>[6x]TESDRIAGIFNIPAGIIPTGNVLSTIEVCAHRCIFDFFKQIRSDDNSLYSAQFDILLGTYCNTLNFVRFLELGLSVACICTKFPELAYVRDGVIQFEVQQPMIARDGPHPVDQPVHNYMVKRIHKRSLSAAFAIASEALSLLSNTYVDGTEIDSSLRIRAIQQMARNLRTVLDSFERGTADQLLGVLLEKAPPLSLLSPINKFQPEGHLNRVARAALLSDLKRRVCADMFFMTRHAREPRLISAYLSDMVSCTQPSVMVSRITHTNTRGRQVDGVLVTTATLKRQLLQGILQIDDTAADVPVTYGEMVLQGTNLVTALVMGKAVRGMDDVARHLLDITDPNTLNIPSIPPQSNSDSTTAGLPVNARVPADLVIVGDKLVFLEALERRVYQATRVAYPLIGNIDITFIMPMGVFQANSMDRYTRHAGDFSTVSEQDPRQFPPQGIFFYNKDGILTQLTLRDAMGTICHSSLLDVEATLVALRQQHLDRQCYFGVYVAEGTEDTLDVQMGRFMETWADMMPHHPHWVNEHLTILQFIAPSNPRLRFELNPAFDFFVAPGDVDLPGPQRPPEAMPTVNATLRIINGNIPVPLCPISFRDCRGTQLGLGRHTMTPATIKAVKDTFEDRAYPTIFYMLEAVIHGNERNFCALLRLLTQCIRGYWEQSHRVAFVNNFHMLMYITTYLGNGELPEVCINIYRDLLQHVRALRQTITDFTIQGEGHNGETSEALNNILTDDTFIAPILWDCDALIYRDEAARDRLPAIRVSGRNGYQALHFVDMAGHNFQRRDNVLIHGRPVRGDTGQAIPITPHHDREWGILSKIYYYIVIPAFSRGSCCTMGVRYDRLYPALQAVIVPEIPADEEAPTTPEDPRHPLHAHQLVPNSLNVYFHNAHLTVDGDALLTLQELMGDMAERTTAILVSSAPDAGAATATTRNMRIYDGALYHGLIMMAYQAYDETIATGTFFYPVPVNPLFACPEHLASLRGMTNARRVLAKMVPPIPPFLGANHHATIRQPVAYHVTHSKSDFNTLTYSLLGGYFKFTPISLTHQLRTGFHPGIAFTVVRQDRFATEQLLYAERASESYFVGQIQVHHHDAIGGVNFTLTQPRAHVDLGVGYTAVCATAALRCPLTDMGNTAQNLFFSRGGVPMLHDNVTESLRRITASGGRLNPTEPLPIFGGLRPATSAGIAR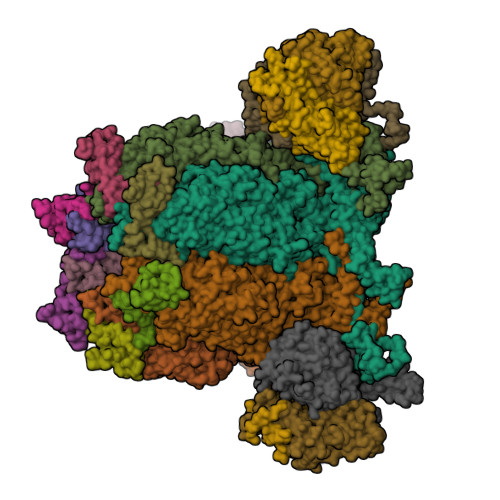GQASVCEFVAMPVSTDLQYFRTACNPRGRASGMLYMGDRDADIEAIMFDHTQSDVAYTDRATLNPWASQKHSYGDRLYNGTYNLTGASPIYSPCFKFFTPAEVNTNCNTLDRLLMEAKAVASQSSTDTEYQFKRPPGSTEMTQDPCGLFQEAYPPLCSSDAAMLRTAHAGETGADEVHLAQYLIRDASPLRGCLPL;>[6x]SNPTTFSVEAIAAYTPVALIRLLNASGPLQPGHRVDIADARSIYTVGAAASAARARANHNANTIRRTAMFAETDPMTWLRPTVGLRRTFNPRII;>AMPFEIEVLLPGELSPAETSALQKCEGKIITFSTLRHRASLVDIALSSYYINGAPPDTLSLLEAYRMRFAAVITRVIPGKLLAHAIGVGTPTPGLFIQNTSPVDLCNGDYICLLPPVYGSADSIRLDSVGLEIVFPLTIPQTLMREIIAKVVARAVEDLNLMFSINEGCLLILALIPRLLALLIPRLLALVTREAAQLIHPEAPMLMLPIYETISSWISTSSRLGDTLGTRAILRVCVFDGPSTVHPGDRTAVIQV[2x];>AMPFEIEVLLPGEISPAETSALQKCEGKIITFSTLRHRASLVDIALSSYYINGAPPDTLSLLEAYRMRFAAVITRVIPGKLLAHAIGVGTPTPGLFIQNTSPVDLCNGDYICLLPPVFGSADEIRLDSVGLEIVFPLTIPQTLMREIIAKVVARAVERTAADVICYNGRRYELETNLQHRDGSDAAIRTLVLNLMFSINEGTTLILTLITRLLRFPIYEAISSWISTSSRLGDTLGTRAILRVCVFDGPSTVHPGDRTAVIQV[2x];>SIQVTPRSIVINRMNNIQINPTSIGNPNNGLHMTYNNAAAAAAAAAAAAAAAAAAAAAAAAAAAAAAAASIQVTPRSIVINRMNNIQINPTSIGNPQVTIRLPLNNFKSTTQLIQQVSLTDFFRPDIEHAGSTVLILRHPTDLPALARHRAPPGRQTERLAEAWGQLLEASRAYVTSLSFIAACRAEEYTDKQAAEANRTAIVSAYGCSRMGARLIRFSECLRAMVQCHVFPHRFISFFGSLLEYTIQDNLCNITAVAKGPQEAARTDKTSTRRVTANIPACVFWDVDKDLHLSADGLKHVFLVFVYTQRRQREGVRLHLALSQLNEQCFGRGIGFLLGARICMYAAYTLIGTIPSESVRYTRRMERFGGYNVPTIWLEGVVWGGTNTWNEC[2x]> 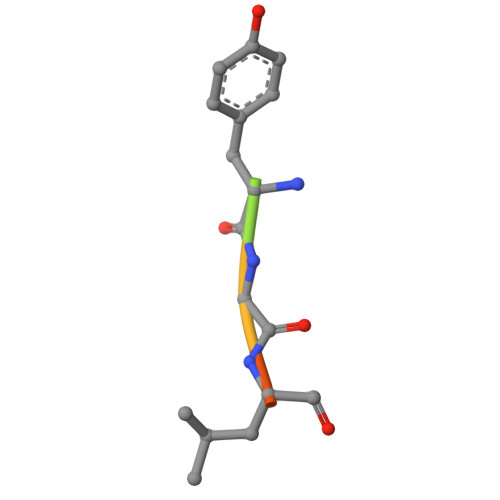SKYGLQD>[2x]MSKLAAFGGPPAVPRDRRHVEWPLVEDEDRKAVIDALDGARLVSNSDGENPVSTLEEQWAGRFGFGHCVAVSTGTAALSLALAALGVGPGDEVIVPALSFIATGLAPVHQMAVPVFAD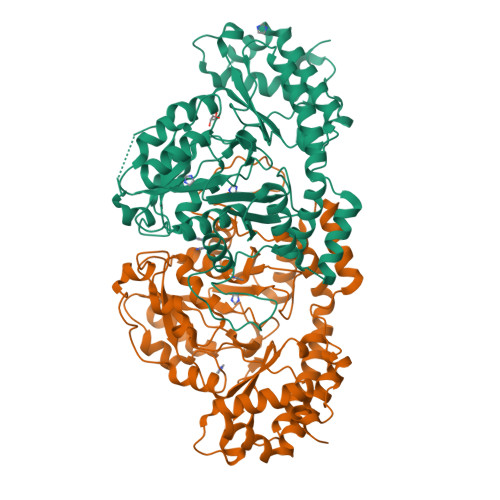VDPVTFNLDPDDVERRITGRTAAIIPVHLHGAPADMDRITAIARRHGLAVIEDAAQAPGATHRGRPVGGIGDAGAFSLQATKNIPTCGEGGLLVTGNAELAESVRRGRQFGEVIESGRERDYVSYGLGWNHKMNALQAAFTSAQLTRFDDYESARQRNVAAFLARLAELPGLRVPTAAPDTTHAWHILRFRFDPAAFGLDGVRPQALRSALRRLLRAEGVPMSQYQLMPLPDQKVFVDRVGFGGGYPWTVTGATGPAAGEDHPVARAVIADSLTLQKRHLHPESGELLHLYADAFEKVWANPDMVATLAGAASGGHHHHHH> KPGFGVGRG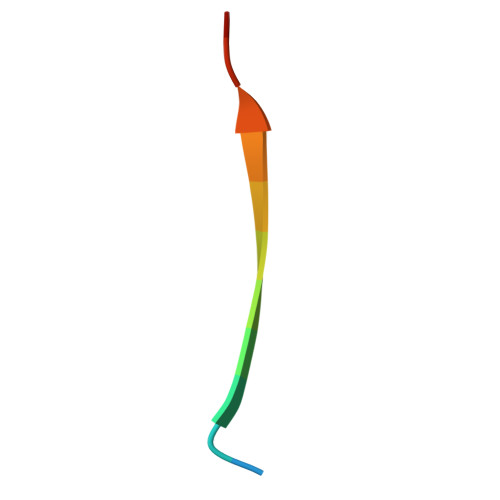LAPR>[2x]MSYYHHHHHH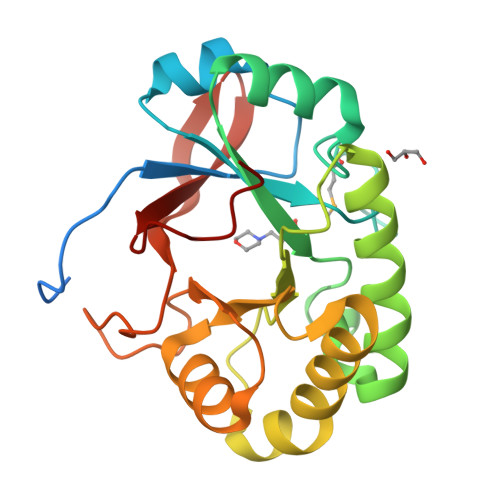LESTSLYKKAGSENLYFQGGSLGTLLDYAAGVIPASQIRAAGAVGAIRYVSDRRPGGAWMLGKPIQLSEARDLSGNGLKIVSCYQYGKGSTADWLGGASAGVQHARRGSELHAAAGGPTSAPIYASIDDNPSYEQYKNQIVPYLRSWESVIGHQRTGVYANSKTIDWAVNDGLGSYFWQHNWGSPKGYTHPAAHLHQVEIDKRKVGGVGVDVNQILKPQFGQWA> GPGSTTSGALFPSLVPGSRGSSTKYLVEFRAGKMSLKGTTVTPDKRKGLVYIQQTDDSLIHFCW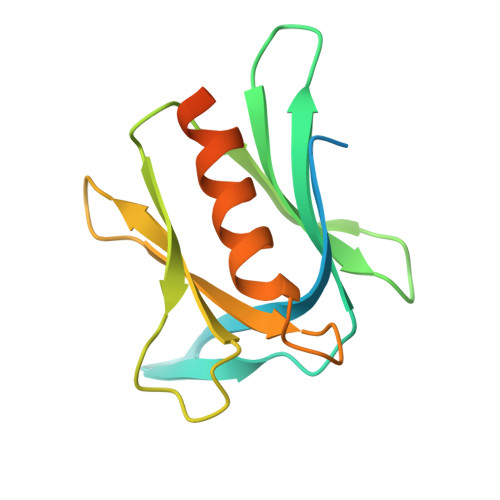KDRTSGTVEDDLIIFPDDCEFKRVPQCPSGRVYVLKFKAGSKRLFFWMQEPKTDQDEEHCRKVNECLNNPPMPGSLGASGSSGHELSAL>[6x]MTNTLQVRLLSENARMPERNHKTDAGYDIFSAETVVLEPQEKAVIKTDVAVSIPEGYVGLLTSRSGVSSKTHLVIETGKIDAGYHGNLGINIKNNAIASNGYITPGVFDIKGEIDLSDA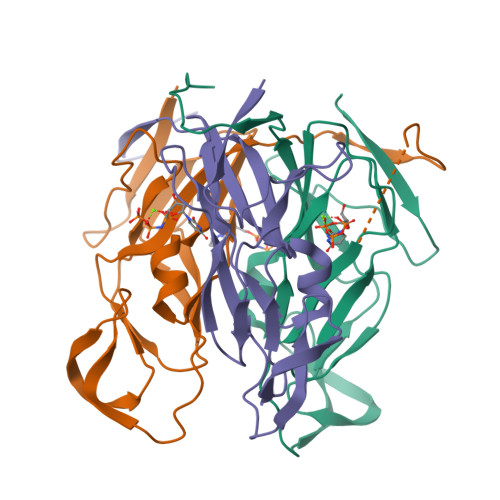IRQYGTYQINEGDKLAQLVIVPIWTPELKQVEEFESVSERGEKGFGSSGV> NGEVEVPKTELEEIQQQCNQVTDDSLESTRRMLNMCEESKEAGIRTLVMLDEQGEQLDRIEEGLDQINQDMKDA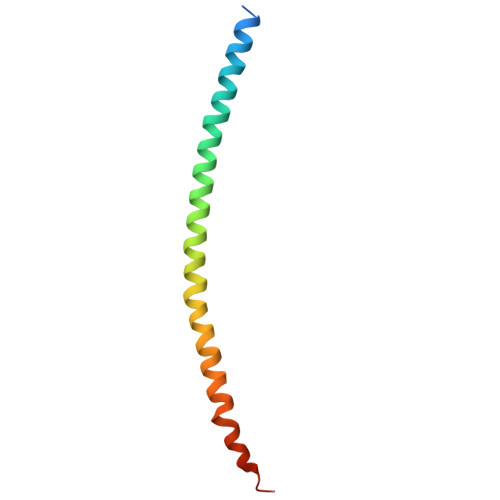EKNLEGMEK> MEGEMQRHIKLTKAQTTPVVLVVGDPGRVDKVKVLCDSYVDLAYNREYKSVECTYKGQKFLCVSHGVGSAGCAICFEELMNNGAKVIIRAGSCGSLQPTQMKRGDICICNAAVREDRVSHLMIYSDFPAVADYEVYATLNQVAEELKVPVFNGISLSSDMYYPHKIIPTRLEDYSKANVAVVEMEVATLMVMGTLRKVKTGGIFIVDGCPLKWDEGDFDNNLVPERL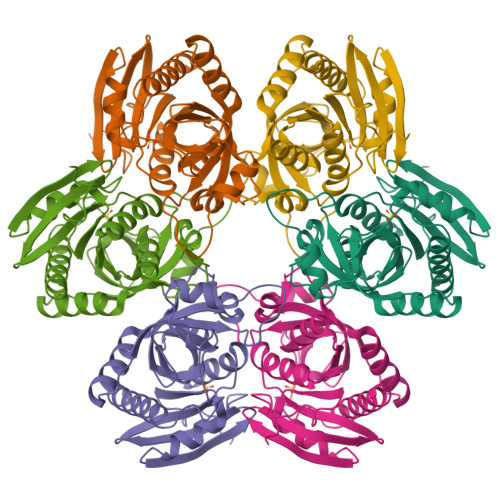ENMIKISLETCARLAKKYLEHHHHHH> MIEEVVAEMIDILAESSKKSIEELARAADNKTTEKAVAEAIEEIARLATAAIQLIEALAKNLASEEFMARAISAIAELAKKAIEAIYRLADNHTTDTFMARAIAAIANLAVTAILAIAALASNHTTEEFMARAISAIAELAKKAIEAIYRLADNHTTDKFMAAAIEAIALLATLAILAIALLASNHTTEKFMARAIMAIAILAAKAIEAIYRLADNHTSPTYIEKAIEAIEKIARKAIKAIEMLAKNITTEEYK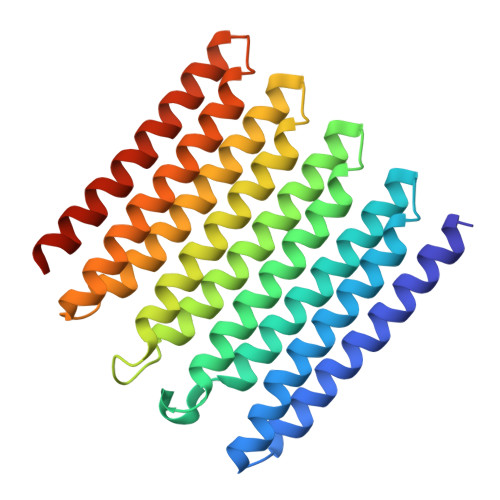EKAKKIIDIIRKLAKMAIKKLEDNRTLEHHHHHH>MKRKKKEEEEEKLIVTREFAKRWRDLSGQNHWKGMLQPLDQDLREYIIHYGEMAQAGYDTFNINTESQFAGASIYSRKDFFAKVGLEIAHPYTKYKVTKFIYATSDIHVPESFLLFPISREGWSKESNWMGYVAVTDDQGTALLGRRDIVVSWRGSVQPLEWVEDFEFGLVNAIKIFGERNDQVQIHQGWYSIYMSQDERSPFTKTNARDQVLREVGRLLEKYKDEEVSITICGHSLGAALATLSATDIVANGYNRPKSRPDKSCPVTAFVFASPRVGDSDFRKLFSGLEDIRVLRTRNLPDVIPIYPPIG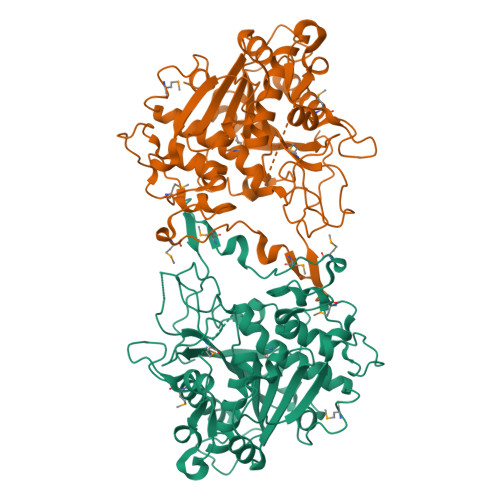YSEVGDEFPIDTRKSPYMKSPGNLATFHCLEGYLHGVAGTQGTNKADLFRLDVERAIGLVNKSVDGLKDECMVPGKWRVLKNKGMAQQDDGSWELVDHEIDDNEDLDF[2x]3-chloro-4-({(2R)-4-[4-fluoro-2-(trifluoromethyl)phenyl]-2-methylpiperazin-1-yl}sulfonyl)benzamide | C19 H18 Cl F4 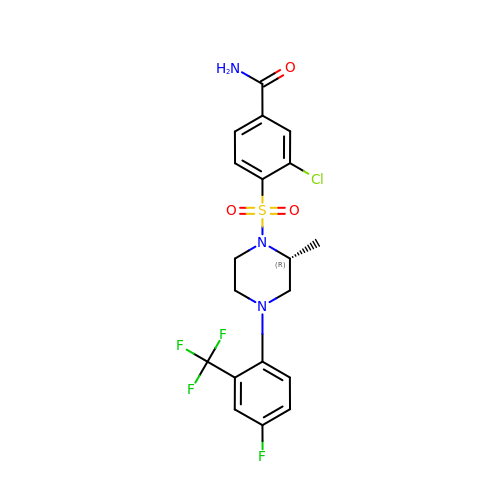N3 O3 S | OMWNFYWEMXUREB-LLVKDONJSA-N>[2x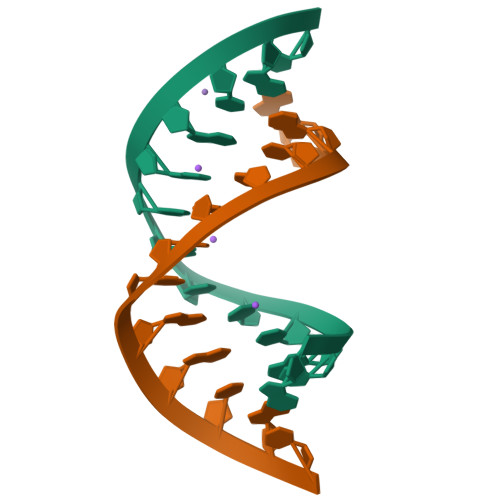]GCGUUUGAAACGC> MQPFDSGHDDLVHDVVYDFYGRHVATCSSDQHI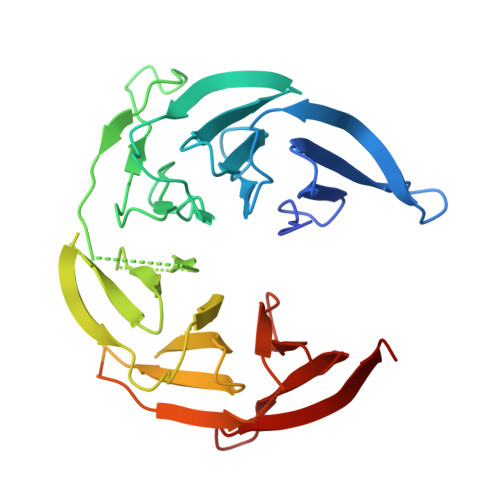KVFKLDKDTSNWELSDSWRAHDSSIVAIDWASPEYGRIIASASYDKTVKLWEEDPDQEECSGRRWNKLCTLNDSKGSLYSVKFAPAHLGLKLACLGNDGILRLYDALEPSDLRSWTLTSEMKVLSIPPANHLQSDFCLSWCPSRFSPEKLAVSALEQAIIYQRGKDGKLHVAAKLPGHKSLIRSISWAPSIGRWYQLIATGCKDGRIRIFKITEKLSPLASEESLTNSNMFDNSADVDMDAQGRSDSNTEEKAELQSNLQVELLSEHDDHNGEVWSVSWNLTGTILSSAGDDGKVRLWKATYSNEFKCMSVITAQQ> GLGQMGSSSTDNTVRETVGAATSRDALPNTEASGPTHSKEIPALTAVETGATNPLVPSDTVQTRHVVQHRSRSESSIESFFARGACVTIMTVDNPASTTNKDKLFAVWKITYKDTVQLRRKLEFFTYSRFDMELTFVVTANFTETNNGHALNQVYQIMYVPPGAPVPEKWDDYTWQTSSNPSIFYTYGTAPARISVPYVG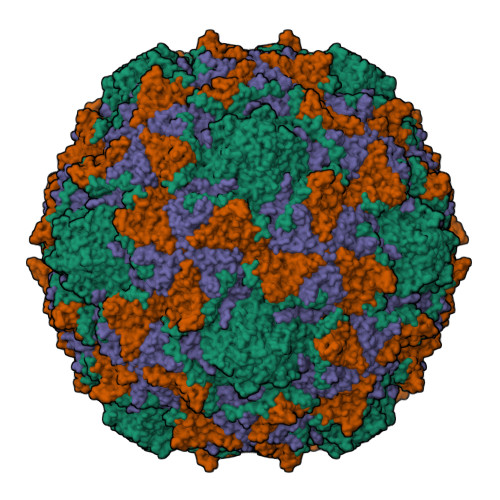ISNAYSHFYDGFSKVPLKDQSAALGDSLYGAASLNDFGILAVRVVNDHNPTKVTSKIRVYLKPKHIRVWCPRPPRAVAYYGPGVDYKDGTLTPLSTKDLTTY;> SPNIEACGYSDRVLQLTLGNSTITTQEAANSVVAYGRWPEYLRDSEANPVDQPTEPDVAACRFYTLDTVSWTKESRGWWWKLPDALRDMGLFGQNMYYHYLGRSGYTVHVQCNASKFHQGALGVFAVPEMCLAGDSNTTTMHTSYQNANPGEKGGTFTGTFTPDNNQTSPARRFCPVDYLLGNGTLLGNAFVFPHQIINLRTNNCATLVLPYVNSLSIDSMVKHNNWGIAILPLAPLNFASESSPEIPITLTIAPMCCEFNGLRNITLPRLQ;> GLPVMNTPGSNQYLTADNFQSPCALPEFDVTPPIDIPGEVKNMMELAEIDTMIPFDLSATKKNTMEMYRVRLSDKPHTDDPILCLSLSPASDPRLSHTMLGEILNYYTHWAGSLKFTFLFCGSMMATGKLLVSYAPPGADPPKKRKEAMLGTHVIWDIGLQSSCTMVVPWISNTTYRQTIDDSFTEGGYISVFYQTRIVVPLSTPREMDILGFVSACNDFSVRLLRDTTHIEQKALA;> GAQVSSQKVGAHENSNRAYGGSTINYTTINYYRDSASNAASKQDFSQDPSKFTEPIKDVLIKTAPMLN>CG[2x];>C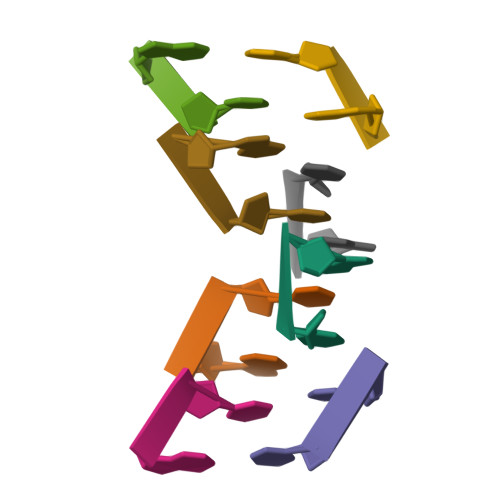GCG[2x]> GAMVSRSTHLVGQDGLCLDVIGGYSDNHVPTQLWPCGPQNNQLWTIQADGTIRTMGKCLVPNGHDPGSYTMIDDCNKADPNDKTWKLYPDGTLTHVRSSLVLTSQGTGAYAITTIETNTSAPTQSWGTAD

Here, we report the discovery and characterization of Cucumis melo agglutinin (CMA1), a new R-type lectin from melon. CMA1 comprises 291 amino acids and is predicted to fold into two linked β-trefoil domains belonging to carbohydrate-binding module family 13 (CBM13) and placing it into the group of R-type lectins. In contrast to other R-type lectins such as ricin, it lacks a catalytic domain. We thus conclude that CMA1 is highly specific for C2-substituted galactose.

Finally, in the presence of 20% PEG 8K, 0.2 M MgCl2, and 0.1 M Tris HCl pH 8.5, single diamond-shaped crystals were obtained after 1–2 days for the N-terminal domain. High-resolution diffraction of the crystals allowed us to solve the CMA1-Nter structure in complex with LacNAc at 1.3 Å and GalNAc at 1.55 Å (see data and refinement statistics in Table 1). All residues of the N-terminal construct (Val6 to Asp132) could be modelled, and unambiguous electron density permitted us to locate and model four cation binding sites (three in each structure) and one sugar binding site. However, only the alpha site was found occupied with a carbohydrate here. It is found in a shallow groove, supporting our data on the lack of a distinct distal binding specificity. We report a tight coordination of the O3 and O4 hydroxy groups of the galactose residue involving Asp21, Asn43, and Gln41 side chains, as well as the Gly24 main chain nitrogen. CH−π stacking and hydrophobic interactions occur between the aromatic ring of Trp36 and the alpha face of the ring as well as the hydroxymethyl moiety of the galactose residue, additionally ensuring specificity for galactoside over glucoside as an equatorial conformation of the O4 hydroxy group would lead to steric clashes and loss of strong hydrogen bonding. Further, beyond the C2 position of galactose, a cavity filled with coordinated water molecules hinted at the binding mode for C2-substituted galactose. Notably, the seemingly inactive beta site was found to be occupied by a cadmium ion, supporting our ITC and SPR data where no multivalent binding effects were observed for the single-domain N-terminal construct. Inhibiting binding of CMA1 to the GalNAc chip through a dilution series of N-acetyllactosamine (LacNAc) via multicycle kinetics allowed us to derive an IC50 of 1.4 µM.N-(4-{[4-(cyclohexylamino)-1-(3-fluorophenyl)-2-oxo-1,3,8-triazaspiro[4.5]dec-3-en-8-yl]methyl}phenyl)acetamide 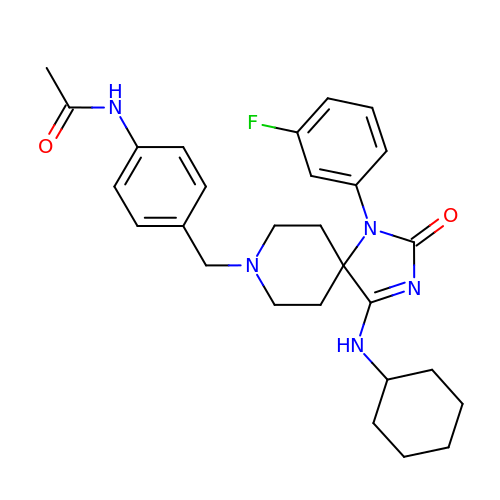| C28 H34 F N5 O2 | VXIOVOURIXSOTD-UHFFFAOYSA-N N-(4-{[2-(2-amino-4-oxo-4,7-dihydro-3H-pyrrolo[2,3-d]pyrimidin-6-yl)ethyl]amino}benzene-1-carbonyl)-L-glutamic 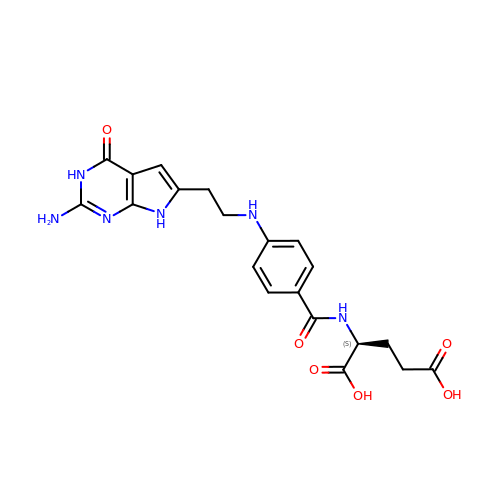acid | C20 H22 N6 O6 | UFNWIIALSMNORN-AWEZNQCLSA-N>[2x]GASLAQPPLP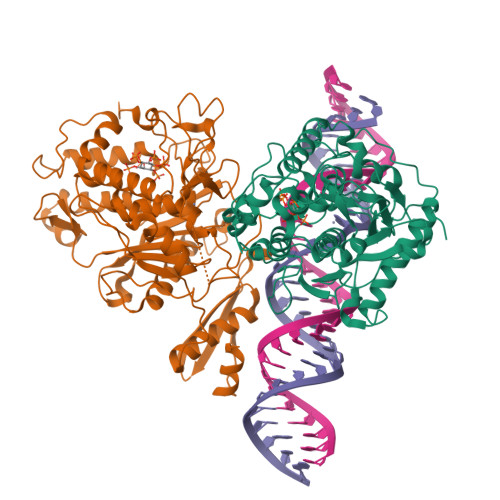VLPPFPPPSGKNPVMILNELRPGLKYDFLSESGESHAKSFVMSVVVDGQFFEGSGRNKKLAKARAAQSALAAIFNLHLDQTPSRQPIPSEGLQLHLPQVLADAVSRLVLGKFGDLTDNFSSPHARRKVLAGVVMTTGTDVKDAKVISVSTGTKCINGEYMSDRGLALNDCHAEIISRRSLLRFLYTQLELYLNNKDDQKRSIFQKSERGGFRLKENVQFHLYISTSPCGDARIFSPHEPILEEPADRHPNRKARGQLRTKIESGQGTIPVRSNASIQTWDGVLQGERLLTMSCSDKIARWNVVGIQGSLLSIFVEPIYFSSIILGSLYHGDHLSRAMYQRISNIEDLPPLYTLNKPLLSGISNAEARQPGKAPNFSVNWTVGDSAIEVINATTGKDELGRASRLCKHALYCRWMRVHGKVPSHLLRSKITKPNVYHESKLAAKEYQAAKARLFTAFIKAGLGAWVEKPTEQDQFSLTP> MDINIDDILAELDKETTAVDSTKITQGSSSTTHRDANTIVGSSLDLNDKTQIYVSPQQDFSDLMKSWKNERCSPELLPYPHQLMKRLLNRISMQSQLIENISMGFLDMQNASNANPPMPNESKLPLLCMETELERLKFVIRSYIRCRLSKIDKFSLYLRQLNEDENSLISLTDLLSKDEIKYHDTHSLIWLKLVNDSILKYMPEELQAINDTEGSVNMIDEPDWNKFVFIHVNG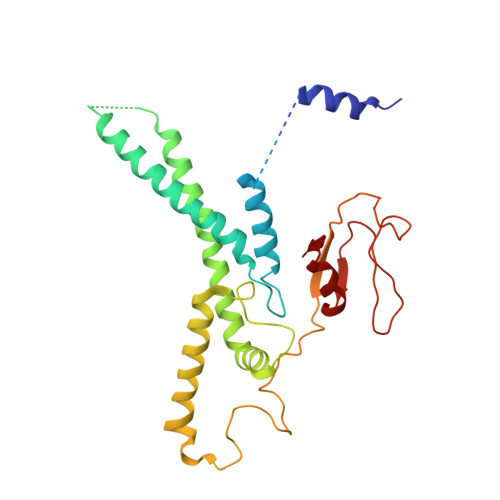PPDGKWNEDPLLQENEFGKPCYTVTIPDLKEEVELTIGSIYVMRYEVIRDLLRDDKVALI>[2x]MGSSHHHHHHSSGPQQGLRQYKTVKVKAPFPMQPIKVFIYPDRDFKITDFGAVPGGEVDNTKAIAAAIDACNKAGGGRVVVPAGIWLTGPVHFKSNINLCLEEDAVLSFTDNPEDYLPAVMTSWEGLECYNYSPLLYAFECENVAISGKGTLQPKMGTWKVWFKRPAPHLQALKELYTKASTNVPVIERQMAIGENHLRPHLIHFNRCKNVMLDGFKIRE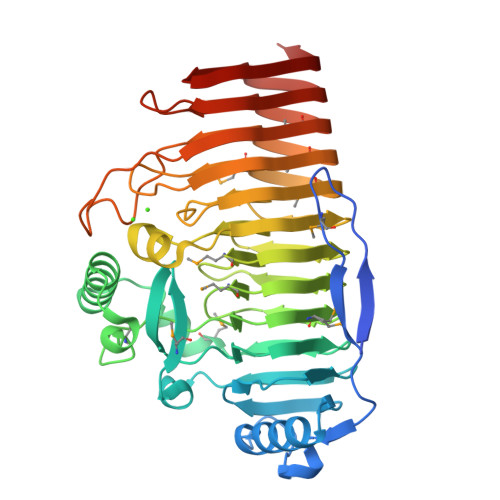SPFWTIHLYMCDGGIVRNLDVRAHGHNNDGIDFEMSRNFLVEDCSFDQGDDAVVIKAGRNQDAWRLNTPCENIVIRNCRILKGHTLLGIGSEISGGIRNIYMHDCTAPNSVMRLFFVKTNHRRGGFIENIYMKNVASGTAQRVLEIDTEVLYQWKDLVPTYEKRITRIDGIYMDKVTCESADAVYELKGNAELPVKNVRIKDVKVGSVKKFVKKVSNVENVVEKNVTYSQKD> MSIDNVLREFLDYKIIALLHDPPNKAWVITGRARNLTQQLSNIRASRKHEKVAKYIINQLFGKNYSEKVDNADKLASSIDRYLGSIVYKERSLFENRSIFLKNILLSNIQRDIGNLFPKDKSKLDNLILEYKKLLNVINKTNLILKYQLFYLIYELVWIDSKYENTPSDTRNPTHTIFDHLYATAAMMNWILSLEKEAKGYLLGIDTIGVADFISKGRKTRDLWISSYLVSALLWYVITWFIEEYGPDVILFPSLRFNQFYAFYLLEKLRKEGVSEDVIDEIKELITKYIFNGDDLFENLKIPPYPIIPGRITLILPGLIREGEEYKKVQDDNCFISKVKERYNEGWRKLIEGLRCYSERKREDGFWNLVCRVLKLTEDLLQTTPLNIRVKQVSVTEDEIFNNNKLRSDSWKIYDNKYRQLVSEFKKSKLVKVTPESRLKLFELTKFDKLPQIGEKSKRGYEFCTSCGVLPAVVIMPKEDELEKKLIDLGIARDEKDVRSIKNMISPGERLCPWCLVKRALGAEPRLMRILLLGDLYSVEKIVNEIVSRDVKIEIPSTSDIASIKTFEEMIEKKNEICEDLKEEE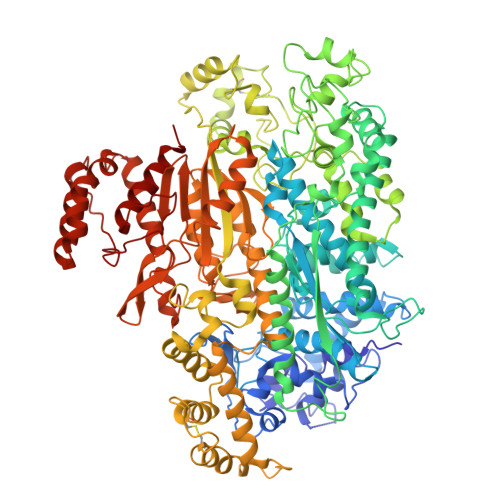VCEKPSESVLSMWQWFNKNYYNGINLTIDPEEYWFSEKRRRYYFSVFRRHRITFPSPYYALVRADSDYLGDLLEGKLTPYLAGIIDSGDYANISEKKEEVNKLLEEYLVNAGSGSIVDYVKTVLKCIRENLNKCSCAEKIYSNEVAKVMFRVNVEKANVEEEVKNSLEYFETILNEGRIIVTPAWHVSISSALNRGLLVELELVNKHKGFVIYAGGDDLLAMLPVDEVLDFIKESRRAFAGFGTEKLGNMCLENGFVRINNAYYPSLPIVGRSYSVIIAHYADPLFFVINDSYNLLEEGKEIIRYRVMYNGEYKDAKKDVAIFRYQGLTSVIPLSLKRPIVSSVSDFNEIASIIDVILELKKRIDEGRISVSLLYDYEKYKHLIVASDEKYLTEFLVKDWIKRNSLRKHVEFTIDEKLYGVRLTIENYPIKIPNDLISNIVYTLRIIYGGEK>MNQSCPNKTSFKIAFIQARWHADIVDEARKSFVAELAAKTGGSVEVEIFDVPGAYEIPLHAKTLARTGRYAAIVGAAFVIDGGIYRHDFVATAVINGMMQVQLETEVPVLSVVLTPHHFHESKEHHDFFHAHFKVKGV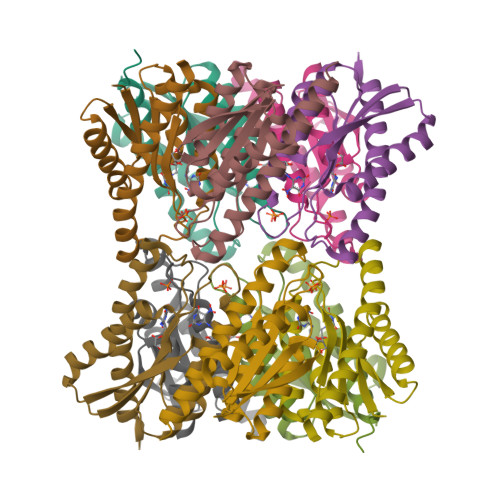EAAHAALQIVSERSRIAALV[5x]>[6x]MAPFEIPDRYKKPAKMLHEICIAESGASEEQLRTCLDGTVPTAPAAKCYIHCLFDKIDVVDEATGRILLDRLLYIIPDDVKAAVDHLT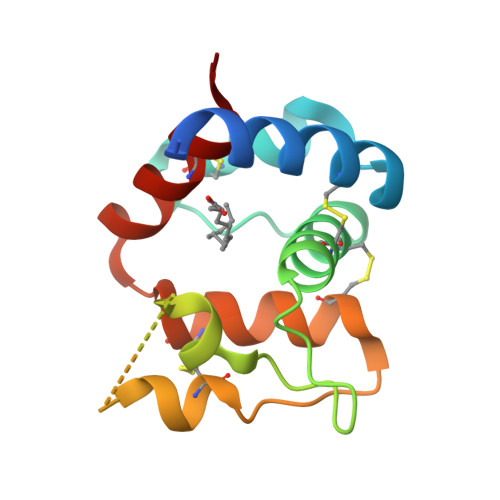RECSHIVTPDKCETAYETVKCYFNAHDEVIKFCHLLVLE> MFPFALLYVLSVSFRKIFILQLVGLVLTYDFTNCDFEKIKAAYLSTISKDLITYMSGTKSTEFQNTVSCSNRPHCLTEIQSLTFNPTAGCASLAKEMFAMKTKAALAIWCPGYSETQINATQAMKSVTTNKCLEQVSQLQGLWRRFNRPLLKQQGTKHHHHHH;> GSHMESGNAQDGDLEDADADDHSFWCHSQLEVDGSQHLLTCAFNDSDINTANLEFQICGALLRVKCLTLNKLQDIYFIKTSEFLLIGSSNICVKLGQKNLTCKNMAIN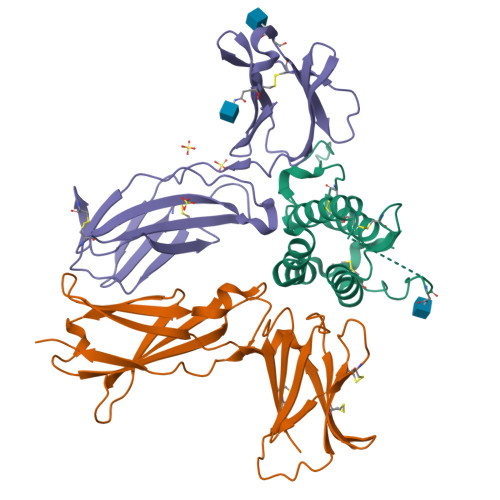TIVKAEAPSDLKVVYRKEANDFLVTFNAPHLKKKYLKKVKHDVAYRPARGESNWTHVSLFHTRTTIPQRKLRPKAMYEIKVRSIPHNDYFKGFWSEWSPSSTFETPEPKNQGGWD;> MGRLVLLWGAAVFLLGGWMALGQGGAAEGVQIQIIYFNLETVQVTWNASKYSRTNLTFHYRFNGDEAYDQCTNYLLQEGHTSGCLLDAEQRDDILYFSIRNGTHPVFTASRWMVYYLKPSSPKHVRFSWHQDAVTVTCSDLSYGDLLYEVQYRSPFDTEWQSKQENTCNVTIEGLDAEKCYSFWVRVKAMEDVYGPDTYPSDWSEVTCWQRGEIRDACAETGTKHHHHHH> MALSRPLPSWLRKPLGKASEISTVQRLVRQYGIHTICEEGRCPNRGECYGQKTATFLLLGPTCTRACAFCQVEKGHAPAAVDPEEPTKIAAAVATLGLRYVVLTSVARDDLPDQGAGQFVATMAAIRQRCPGTEIEVLSPDFRMDRGRLSQRDCIAQIVAAQPACYNHNLETVRRLQGPVRRGATYESSLRVLATVKELNPDIPTKSGLMLGLGETEAEII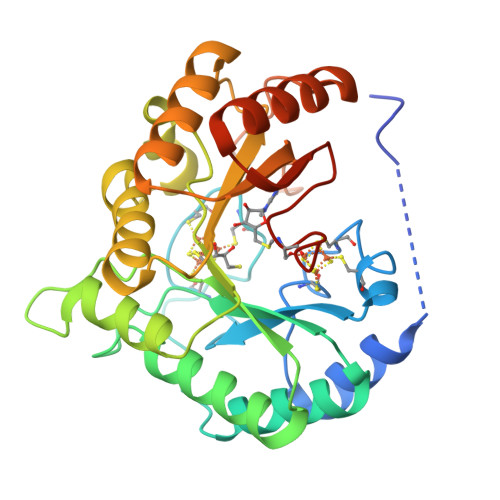ETLKDLRRVGCDRLTLGQYLPPSLSHLPVVKYWTPEEFNTLGNIARELGFSHVRSGPLVRSSYHAAEGGHHHHHH>SREDLRAWLTRNRFPRVGGVSESTVQWEGVVFTVSNESVPRWVMAQIQPAYMGLVATQASLAAAEAVAAVARRRGIEVHGPLQVADPNDPAASRSQVALLLSELRRAGCREIAVDLTGGKLPMSLGAFMAAEEAGVASLYVATDFDKHLKVPDMRTATLRQISQPE[2x]

Prokaryotic type III CRISPR–Cas systems provide immunity against viruses and plasmids using CRISPR-associated Rossman fold (CARF) protein effectors. We studied WP_013033759 (hereafter named Cam1) from the halophilic Gram-negative chromatiaceae Nitrosococcus halophilus Nc4, which contains a CARF domain fused to a transmembrane domain that does not seem to be capable of degrading nucleic acids, as is the case for all the previously characterized CARF effectors. N. halophilus Cam1 (hereafter NhCam1) has a molecular mass of 22.3 kDa and contains 206 amino acids, with an N-terminal transmembrane helix (TMH) predicted to be 24 amino acids in length by deepTMHMM26 followed by an equally short linker (L1) and a C-terminal intracellular CARF domain. Here we investigated the structure and function of Cam1, a CARF effector that lacks a nuclease domain, but contains a TMH domain that promotes the formation of a tetrameric pore that is required to provide immunity through membrane depolarization and growth arrest of the infected cell (Supplementary Discussion).

We found that cA4 binds to the CARF domain of NhCam1 with a dissociation constant (Kd) of 12 nM and a stoichiometry of one ligand per CARF domain dimer (n = 0.5), whereas no binding is observed on addition of cA6, cA2 or cA3. By contrast, the 2.1 Å X-ray structure of NhCam1-CARF bound to cA4 shows that it adopts a dimeric fold with no domain swap between the monomers. Loop L2 adopts different conformations in each monomer of the NhCam1-CARF dimer in the complex, with the N and C termini being in close proximity in one monomer but far apart in the other monomer, owing to crystal packing forces. The bound cA4 is positioned over a platform generated from both monomers, and is further capped by a pair of L2 loops, thereby encapsulating the ligand. The bound cA4 complex is stabilized by hydrogen-bond interactions between N1 nitrogens of A2 and A4 and the Thr97 side chains of the CARF domain, hydrogen-bond interactions involving the backbone phosphates of bound cA4, as well as hydrophobic contacts between the adenosine rings and non-polar side chains of the CARF domain. The overall topology, hydrogen-bonding and hydrophobic interactions involving second messenger binding in NhCam1 show similarities with cA4-bound TsCard13, but not with TsCsm65 or SiCsx14. Alanine substitutions of amino acids involved in hydrogen bonds with cA4—T97A, S75A/N76A and Y180A/T183A—reduced ligand affinity from 17 nM to 3.74 µM, 4.0 µM and 4.5 µM, respectively. Triple alanine substitutions of amino acids involved in hydrophobic contacts with the ligand—K160A/F185A/L189A and V79A/P192A/M194A—resulted in a complete absence of ligand binding, and a reduction of binding affinity to 2.1 µM, respectively. Analysis of single alanine mutants showed that K160, F185 and L189 are all essential for NhCam1 function in vivo, and are therefore presumably important for cA4 binding during the type III-A immune response.>[2x]HGGEAHMVPMDKTLKEFGADVQWDDYAQLFTLIKDGAYVKVKPGAQTAIVNGQPLALQVPVVMKDNKAWVSDTFINDVFQSGLDQTFQVEKRPHPLNALTADEIKQAVEIVKASADFKPNTRFTEISLLPPDKEAVWAFALENKPVDQPRKADVIMLDGKHIIEAVVDLQNNKLLSWQPIKDAHGMVLLDDFASVQNIINNSEEFAAAVKKRGITDAKKVITTPLTVGYFDGKDGLKQDARLLKVISYLDVGDGNYWAHPIENLVAVVDLEQKKIVKIEEGPVVPVPMTAR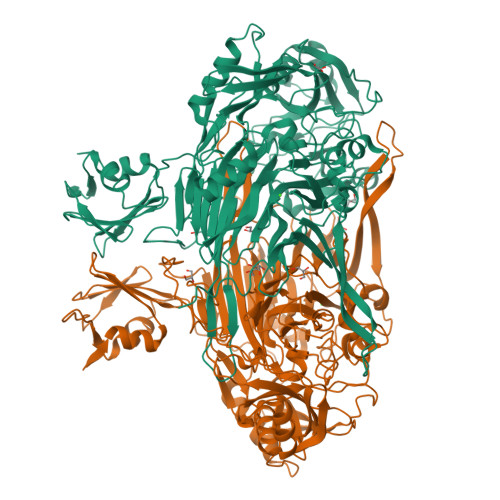PFDGRDRVAPAVKPMQIIEPEGKNYTITGDMIHWRNWDFHLSMNSRVGPMISTVTYNDNGTKRKVMYEGSLGGMIVPYGDPDIGWYFKAYLDSGDYGMGTLTSPIARGKDAPSNAVLLNETIADYTGVPMEIPRAIAVFERYAGPEYKHQEMGQPNVSTERRELVVRWISTVGNYDYIFDWIFHENGTIGIDAGATGIEAVKGVKAKTMHDETAKDDTRYGTLIDHNIVGTTHQHIYNFRLDLDVDGENNSLVAMDPVVKPNTAGGPRTSTMQVNQYNIGNQQDAAQKFDPGTIRLLSNPNKENRMGNPVSYQIIPYAGGTHPVAKGAQFAPDEWIYHRLSFMDKQLWVTRYHPGERFPEGKYPNRSTHDTGLGQYSKDNESLDNTDAVVWMTTGTTHVARAEEWPIMPTEWVHTLLKPWNFFDETPTLGALKKDK>NSAMLKTLLTSDVIQVVSQAKDWRDAIAISCQPLIDNGAVEARYVEAIYRSHEAIGPYYVVGPGIAMPHARPEDGVNRLSLALTVITEGVTFNAEGNDPVKLLIVLAAT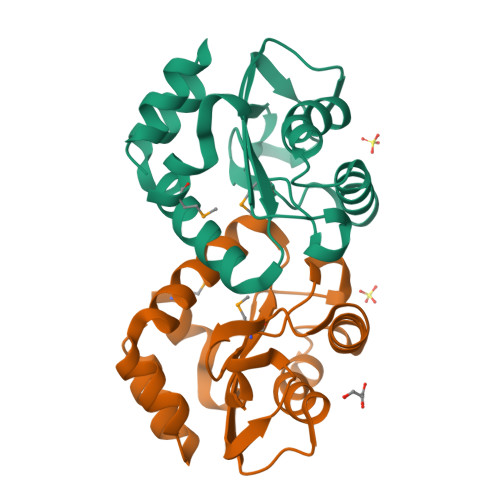DSNSHIEAISQLAQLFDTASDVQALLNAKTPQDILSVIARY[2x]>[2x]VLTEGNPRWEQTHLRYRIENYTPDLPRADVD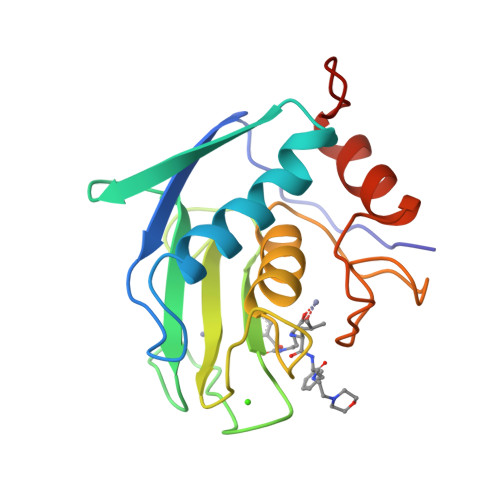HAIEKAFQLWSDVTPLTFTKVSEGQADIMISFVRGDHRDNSPFDGPGGNLAHAFDPGPGIGGDAHFDEDERWTNNFREYNLHRVAAHELGHSLGLSHSTDIGALMYPSYTFSGDVQLAQDDIDGIQAIYGRSQNPVQP> THWFHRNPLKATAPVSFNYYGVVTGPSASKICNDLRSSRARLLELFTDLSCNPEMMKNAADSYFSLLQGFINSLDESTQESKLRYIQNFKWTDTLQGQVPSAQQDAVFELISMGFNVALWYTKYASRLAGKENITEDEAKEVHRSLKIAAGIFKHLKESHLPKLITPAEKGRDLESRLIEAYVIQCQAEAQEVTIARAIELKHAPGLIAALAYETANFYQKADHTLSSLEPAYSAKWRKYLHLKMCFYTAYAYCYHGETLLASDKCGEAIRSLQEAEKLYAKAEALCKEYGETKGPGPTVKPSGHLFFRKLGNLVKNTLEKCQRENGFIYFQKIPTEAPQLELKANYGLVEPIPFEFPPTSVQWTPETLAAFDL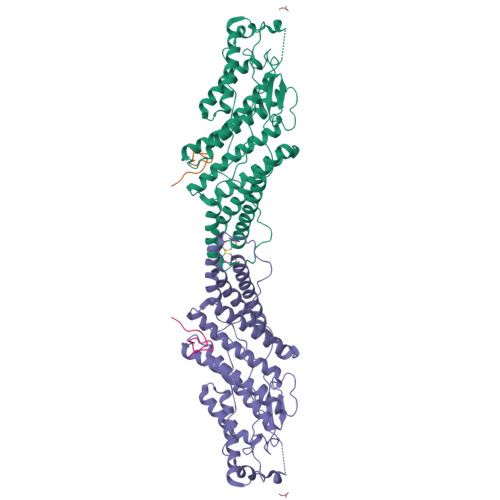TKRPKDDSTKPKPEEEVKPVKEPDIKPQKDTGCYIS;> TKNKDGVLVDEFGLPQIPAS>GVVGSDARSRGRVPGYASSSLYRESGIISARQLALLQRMLPRLRLEQLFRCEWLQQRLARGLALGREEVRQI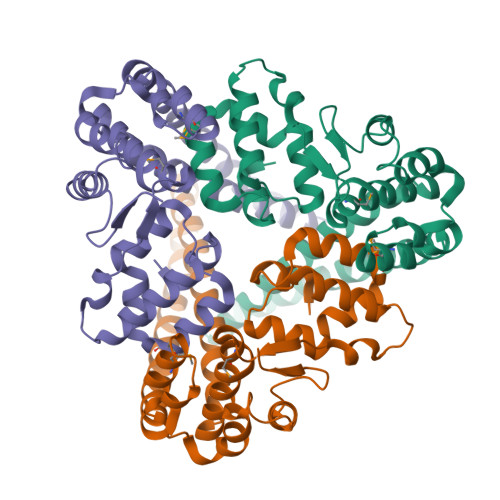LLCAAQDDDGWCAELGDRVNLAVPQSMIDWVLLPVYGWWESLLDQAIPGWRLSLVELETQSRQLRIKSEFWSRVAELEPEQAREELARVAKCQARTQEQVAELAGKLETASALAKSAWPNWQRGMATLLASGGLAGFEPIPEVLECLWQPLCRLDDDVGAADAVQAWLHERNLCQAQDHFYWQS[3x]> MLGILNKMFDPTKRTLNRYEKIANDIDAIRGDYENLSDDALKHKTIEFKERLEKGATTDDLLVEAFAVVREASRRVTGMFPFKVQLMGGVALHDGNIAEMKTGEGKTLTSTLPVYLNALTGKGVHVVTVNEYLASRDAEQMGKIFEFLGLTVGLNLNSMSKDEKREAYAADITYSTNNELGFDYLRDNMVLYKEQMVQRPLHFAVIDQVDSILIDEARTPLIISGQAAKSTKLYVQANAFVRTLKAEKDYTYDIKTKAVQLTEEGMTKAEKAFGIDNLFDVKHVALNHHINQALKAHVAMQKDVDYVVEDGQVVIVDSFTGRLMKGRRYSEGLHQAIEAKEGLEIQNESMTLATITFQNYFRMYEKLAGMTGTAKTEEEEFRNIYNMQVVTIPTNRPVVRDDRPDLIYRTMEGKFKAVAEDVAQRYMTGQPVLVGTVAVETSELISKLLKNKGIPHQVLNAKNHEREAQIIEEAGQKGAVTIATNMAGKGTDIKLGEGVKELGGLAVVGTERHESRRIDNQLRGRSGRQGDPGITQFYLSMEDELMRRFGAERTMAMLDRFGMDDSTPIQSKMVSRAVESSQKRVEGNNFDSRKQLLQYDDVLRQQREVIYKQRFEVIDSENLREIVENMIKSSLERAIAAYTPREELPEEWKLDGLVDLINTTYLDEGALEKSDIFGKEPDEMLELIMDRIITKYNEKEEQFGKEQMREFEKVIVLRAVDSKWMDHIDAMDQLRQGIHLRAYAQTNPLREYQMEGFAMFEHMIESIEDEVAKFVMKAEIENNLEREEVVQGQTTAHQPQEGDDNK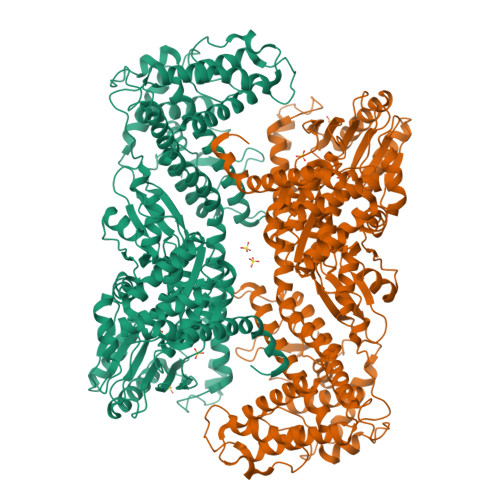KAKKAPVRKVVDIGRNAPCHCGSGKKYKNCCGRTE>SMNYFVGNSLGVNLTGIEKAIINRLNLFKEMGRPAQCVFLSWNRYLYRNAQNYITSSDYINMYDFFQEATYLERNEPFDWLSYWTDECHYTLKHVENSHDFRIY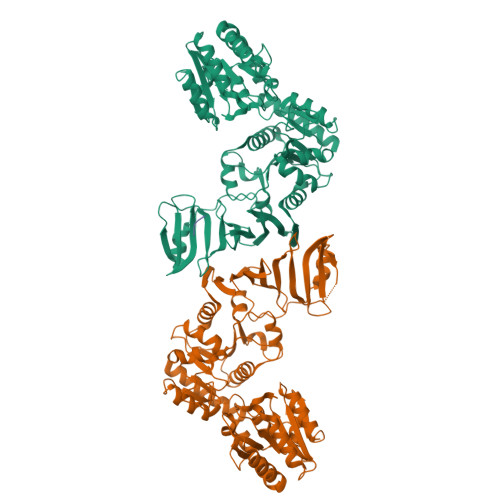DQERFLMYAHFQDPKYRILDYVNHFDSQRRKVKRDFYDVRGFLSCSRILVDKQQTLCEFFYNPEGDTKLEKYFSYKDGKPEVQKIIVYYANKQYFFNNETELGAFFIKQLYQHGDLFFSDRNVYTAPIFNLTPESIPVVAVLHSTHIKNIDALDSSPFKNVYKAMFENLSRYRAIIVSTEQQKLDVEKRINHTIPVVNIPVGYSETIDTPVQTLDQRSVKLISVARYSPEKQLHQQIELIKRLVSYVPKIELHMYGFGSESKKLNELIQKYGLENHVYLRGFLSNLDQEYSDAYLSLITSNMEGFSLALLESLAHGVPVISYDIKYGPNELITSDFNGYLITKNDEDALFDKVKYVIDHPEVQQRLSKGSLAKAQQYSKASLIKQWDQFVRLILEHHHHHH[2x];> DSD> MSALFEPYTLKDVTLRNRIAIPPMCQYMAEDGMINDWHHVHLAGLARGGAGLLVV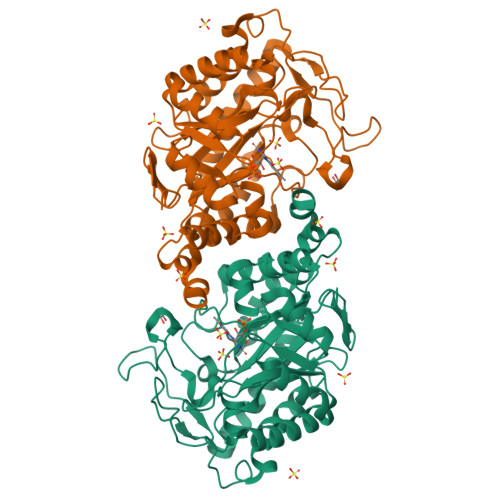EATAVAPEGRITPGCAGIWSDAHAQAFVPVVQAIKAAGSVPGIQIAHAGRKASANRPWEGDDHIAADDTRGWETIAPSAIAFGAHLPKVPREMTLDDIARVKQDFVDAARRARDAGFEWIELHFAHGYLGQSFFSEHSNKRTDAYGGSFDNRSRFLLETLAAVREVWPENLPLTARFGVLEYDGRDEQTLEESIELARRFKAGGLDLLSVSVGFTIPDTNIPWGPAFMGPIAERVRREAKLPVTSAWGFGTPQLAEAALQANQLDLVSVGRAHLADPHWAYFAAKELGVEKASWTLPAPYAHALERYR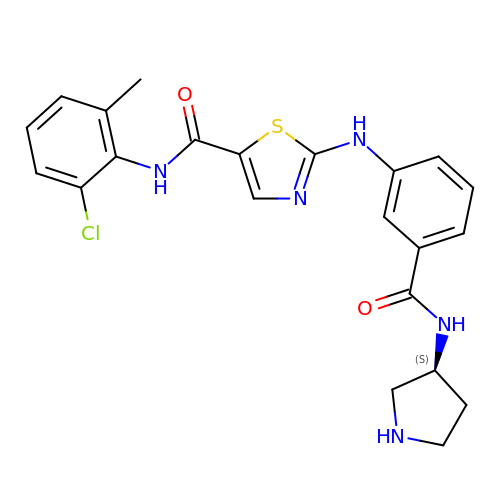~{N}-(2-chloranyl-6-methyl-phenyl)-2-[[3-[[(3~{S})-pyrrolidin-3-yl]carbamoyl]phenyl]amino]-1,3-thiazole-5-carboxamide | C22 H22 Cl N5 O2 S | NFJBJEVYNAEEOP-INIZCTEOSA-N> MPAPLYGADDPRRCSGNSVSEVLDKFRKNYDLIMSLPQETKEEKEFRHCIWLAEKE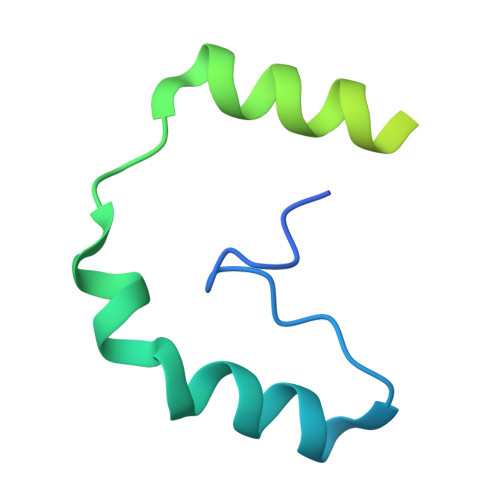ERERIYQTAIRPFRKATYTKFIEIDPRLRDYRSRYAGISNN>[2x]KRVLVVDDEESITSSLSAILEEEGYH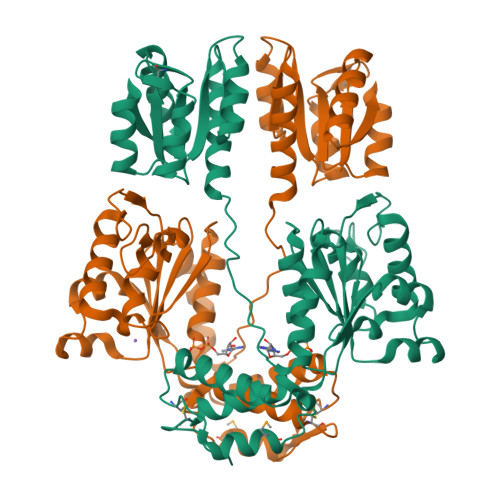PDTAKTLREAEKKIKELFFPVIVLDVWMPDGDGVNFIDFIKENSPDSVVIVITGHGSVDTAVKAIKKGAYEFLEKPFSVERFLLTIKHAFEEYSKKAPPQEEIEFVGEHPKILEIKRLIPKIAKSKAPVLITGESGTGKEIVARLIHRYSGRKGAFVDLNCASIPQELAESELFGHEKGAFTGALTRKKGKLELADQGTLFLDEVGELDQRVQAKLLRVLETGSFTRLGGNQKIEVDIRVISATNKNLEEEIKKGNFREDLYYRLSVFQIYLPPLRERGKDVILLAEYFLKKFAKEYKKNCFELSEETKEYLMKQEWKGNVRELKNLIERAVILCEGEVIKP>XPPGPPGLPGERGLRGEPGPPGPPGPPG[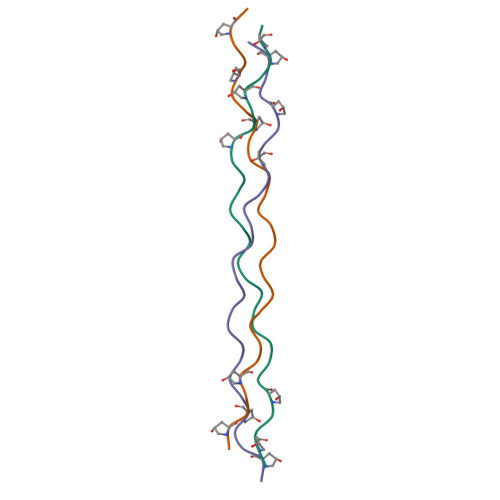3x]The WWE domain is a relatively under-researched domain found in twelve human proteins and characterized by a conserved tryptophan-tryptophan-glutamate (WWE) sequence motif. Six of these WWE domain-containing proteins also contain domains with E3 ubiquitin ligase activity. Here, we present novel crystal structures of the HUWE1, TRIP12, and DTX1 WWE domains in complex with PAR building blocks and their analogs, thus enabling a comprehensive analysis of the PAR binding site structural diversity. A highly conserved feature in all determined structures is the recognition and therefore the interactions involving the adenine ring of the ligands.

Unlike HUWE1, RNF146 and TRIP12 which each possess only one WWE domain, the DTX subfamily is characterized by a tandem-WWE arrangement. In general, the binding of ADPr and ATP to DTX1 was found to be very weak, with affinities of 709 μM and 659 μM, respectively. To visualize the interactions of ATP with the WWE domains, we solved the crystal structures of TRIP12 and DTX1 in complex with ATP. The DTX1-ATP structure has one ATP molecule in the WWE1 domain while WWE2 is unbound, a trend observed with our DTX1-ADP structures. The ATP molecule binds the same way as ADP in the DTX1-ADP structures, with the terminal phosphate group of ATP having no interactions with the protein residues. Taken together, the two ATP co-crystal structures provide a detailed characterization of TRIP12 and DTX1 interaction with ATP and show that the interaction with the ADP moiety of ATP is preserved. A superposition of this structure with our ATP bound structures highlights the conservation of ATP binding to the proteins, with the exception of the terminal phosphate group, which adopts different conformations based on the residues in the interacting loop.

>[2x]GNVARVVVWEWLNEHSRWRPYTATVCHHIENVLKEDARGSVVLGQVDAQLVPYIIDLQSMHQFRQDTGTMRPVRRNFYDPSSAPGKGIVWEWENDGGAWTAYDMDICITIQNAYEKQHPWLDLSSLGFCYLIYFNSMSQMNRQTRRRRRLRRRLDLAYPLTVGSI> GHMSSTPSNQNIIPIIKKESIVSLFEKGIRQDGRKLTDYRPLSITLDYAKKADGSALVKLGTTMVLAGTKLEIDKPYEDTPNQGNLIVNVELLPLAYETFEPGPPDENAIELARVVDRSLRDSKALDLTKLVIEPGKSVWTVWLDVYVLDYGGNVLDACTLASVAALYNTKVYKVEQHSNGIS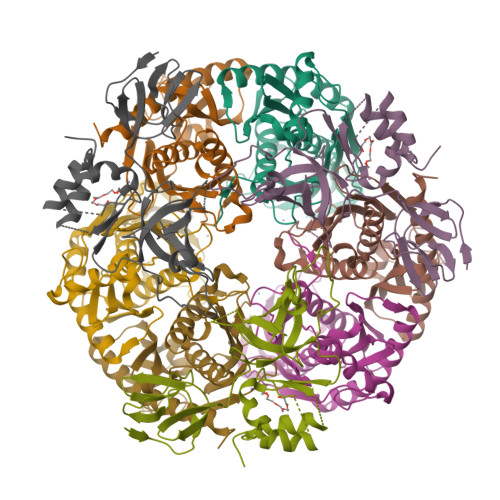VNKNEVVGKLPLNYPVVTISVAKVDKYLVVDPDLDEESIMDAKISFSYTPDLKIVGIQKSGKGSMSLQDIDQAENTARSTAVKLLEELKKHLGI;> GHMREMLQVERPKLILDDGKRTDGRKPDELRSIKIELGVLKNADGSAIFEMGNTKAIAAVYGPKEMHPRHLSLPDRAVLRVRYHMTPFSTDERKNPAPSRREIELSKVIREALESAVLVELFPRTAIDVFTEILQADAGSRLVSLMAASLALADAGIPMRDLIAGVAVGKADGVIILDLNETEAMWGEADMPIAMMPSLNQVTLFQLNGSMTPDEFRQAFDLAVKGINIIYNLEREALKSKYVEFKEEGV;> GHMNMSQSQKIVLQPRSIVVPGELLAEGEFQIPWSPYILKINSKYYSTVVGLFDVKDTQFEVIPLEGSFYYPKINDIVIGLVEDVEIYGWVVDIKAPYKAYLPASNLLGRSINVGEDLRRYLDVGDYVIARIENFDRSIDPVLSVKGKDLGRVSNGIVIDIMPVKVPRVIGKNKSMYETLTSKSGCSIFVANNGRIWATCPSRFSEEILIEAIRKIENESHIKGLTDRIKQFIEEKLGERNASSGETKTNS>GSATATT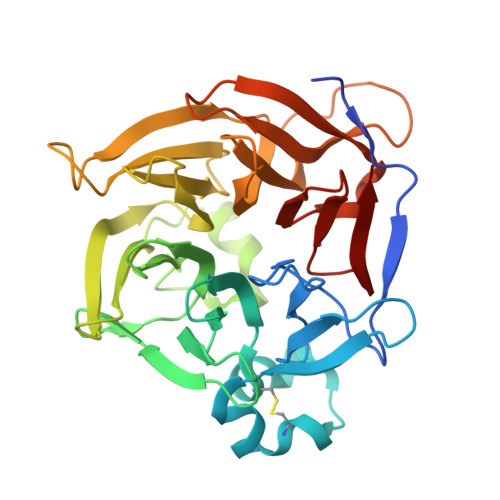RMFKTIDARRSQHLDLGGSLVGPESVAFDGKGRGPYSGVSDGRIMRWNGEAAGWSTYTYSPSYTKNKCAASTLPTVQTESKCGRPLGLRFHYKTGNLYIADAYMGLMRVGPKGGEATVLAMKADGVPLRFTNGVDIDQVTGDVYFTDSSMNYQRSQHEQVTATKDSTGRLMKYDPRTNQVTVLQSNITYPNGVAMSADRTHLIVALTGPCKLMRHWIRGPKTGKSEPFVDLPGYPDNVRPDGKGGYWIALHREKYELPFGPDSHLVAMRVSAGGKLVQQMRGPKSLRPTEVMERKDGKIYMGNVELPYVGVVKSS[12x]>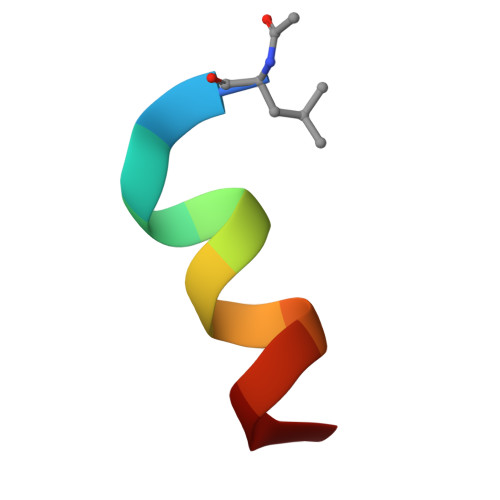 LTFAEYWAQLAS>[12x]MGSSHHHHHHSSGPQQGLRGSTGGPDAPMAVWLQSSLQRIFPQSPAQTAAAL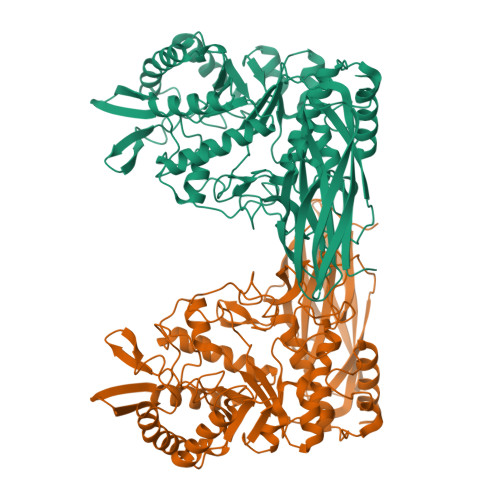ELQAARNSRVSFQVAFRSNMKDQTHISCSTEGAETLHPRVRYVGLVPMPHFNTDVSPEELDGVGYLPGWLPDPLYPVTKTEAHPFESRSFWITLQIPASLSPGIHDFHVRMRWQEGKEEKDKLLHVKVKVSALVLQPRSNFHVTHWWRGEAIALQYETKMFDEQWWKLTRACMKNLIEHGNDVAFIQNFFELRAVFKEPCQMLIVREPSPGKYEFDWSRIKRFVDMCRELGYKKFEWAHLWLYWGVQDAMHVYKKEGNAYKLLWAENLSGTSDTYIHFLKQYLPQLHRFLLKENLLSDSYFHLSDEPWSEHVENYKKARNILRQLAPWMKVMDALSDVRYGREQLTDIPIPIISSDEAYRKEQIPHWVYFCTGPRNKWLNRLYDTPLPKLRMSGWLFYKLKALGFLHWGYNFWYTLDKEQPGDPFTEGAAYAYPGIAYGDPFVVYPGPDGPYDSIRWEVFSESLQDYAILQSAGIQPEDPMLAALHTYEDFPRSEQWINETLKKILEKAK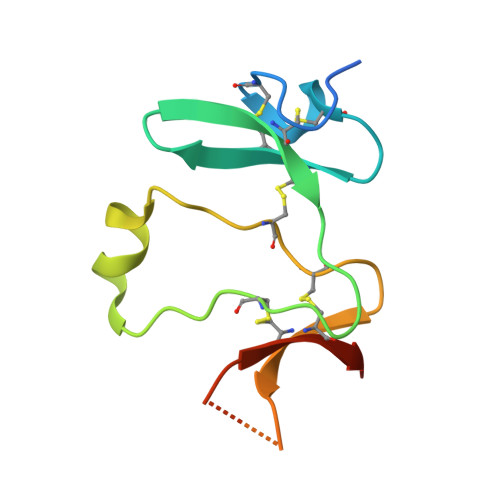> ADPMYHTKGQEGSVCLRSSDCASGLCCARHFWSKICKPVLKEGQVCTKHRRKGSHGLEIFQRCYCGEGLSCRIQKDHHQASNSSRLHTCQRHHHHHH> MAMHPRKDWYELTRATNWTPSYVTEEQLFPERMSGHMGIPLEKWESYDEPYKTSYPEYVSIQREKDAGAYSVKAALERAKIYENSDPGWISTLKSHYGAIAVGEYAAVTGEGRMARFSKAPGNRNMATFGMMDELRHGQLQLFFPHEYCKKDRQFDWAWRAYHSNEWAAIAAKHFFDDIITGRDAISVAIMLTFSFETGFTNMQFLGLAADAAEAGDYTFANLISSIATDESRHAQQGGPALQLLIENGKREEAQKKVDMAIWRAWRLFAVLTGPVMDYYTPLEDRSQSFKEFMYEWIIGQFERSLIDLGLDKPWYWDLFLKDIDELHHSYHMGVWYWRTTAWWNPAAGVTPEERDWLEEKYPGWNKRWGRCWDVITENVLDDRMDLVSPETLPSVCNMSQIPLVGVPGDDWNIEVFSLEHNGRLYHFGSEVD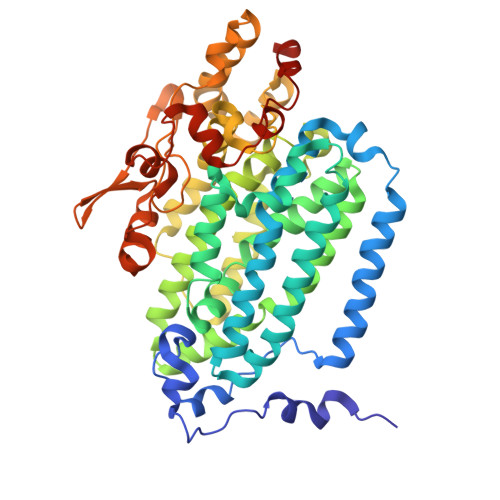RWVFQQDPVQYQNHMNIVDRFLAGQIQPMTLDGALKYMGFQSIEEMGKDAHDFAWADKCKPAMKKSA>[2x]MRKHPQTATKHLFVSGGVASSLGKGLTASSLGQLLTARGLHVTMQKLDPYLNVDPGTMNPFQHGEVFVTEDGAETDLDVGHYERFLDRNLPGSANVTTGQVYSTVIAKERRGEYLGDTVQVIPHITDEIKRRILAMAQPDADGNRPDVVITEIGGTVGDIESQPFLEAARQVRHYLGREDVFFLHVSLVPYLAPSGELKTKPTQHSVAALRSIGITPDALILRCDRDVPEALKNKIALMCDVDIDGVISTPDAPSIYDIPKVLHREELDAFVVRRLNLPFRDVDWTEWDDLLRRVHEPHETVRIALVGKYVELSDAYLSVAEALRAGGFKHRAKVEICWVASDGCETTSGAAAALGDVHGVLIPGGFGIRGIEGKIGAIAYARARGLPVLGLCLGLQCIVIEAARSVGLTNANSAEFDPDTPDPVIATMPDQEEIVAGEADLGGTMRLGSYPAVLEPDSVVAQAYQTTQVSERHRHRYEVNNAYRDKIAESGLRFSGTSPDGHLVEFVEYPPDRHPFVVGTQAHPELKSRPTRPHPLFVAFVGAAIDYKAGELLPVEIPEIPEHTPNGSSHRDGVGQPLPEPASRG

The combined data indicate that 7947882 and 7904688 are prodrugs activated by the EthA monooxygenase, which then target PyrG, a cytidine triphosphate (CTP) synthetase catalyzing the ATP-dependent amination of uridine triphosphate (UTP) to form the essential pyrimidine nucleotide CTP. The crystal structure of PyrG was solved by molecular replacement on a 2.0-Å resolution data set. This structure showed a bidomain enzyme with an N-terminal amidoligase (ALase) domain, also commonly known as the synthetase domain (residues 1–278), connected through an interdomain linker (residues 279–Pro298) to a C-terminal glutamine amidotransferase (GATase) domain (residues 299–552), both domains displaying a Rossmann-like fold. On the other hand, the 34-residue C-terminal extension of M. tuberculosis PyrG, which has no predicted secondary structure or known function, could not be traced due to the lack of supporting electron density, suggesting a high degree of flexibility.

The enzyme, in complex with either UTP, at 2.0-Å resolution, or UTP plus the non-hydrolyzable ATP analog AMP-PCP and the glutamine analog 5-oxo-L-norleucine (3.5 Å), is a homotetramer with crystallographic 222 symmetry, consistent with previous studies reporting positive cooperativity for ATP and UTP due to nucleotide-driven tetramerization. In contrast, in the independent crystal form, grown in the presence of AMP-PCP as well as UTP and the glutamine analog 6-diazo-5-oxo-L-norleucine (L-DON), AMP-PCP lies in the ATP-binding site, as expected, with UTP maintaining the same orientation as above. In addition, a covalent adduct was observed between the Cys393 sulfur and oxonorleucine, as expected from the reaction with L-DON, therefore confirming the role of Cys393 as the catalytic nucleophile within a Gln-hydrolyzing triad that includes His524 and Glu526. In agreement with similar observations made on E. coli PyrG (Endrizzi et al., 2004), a putative ammonia diffusion channel was visualized connecting the glutaminase active site in the C-terminal domain to the synthetase site at the N-terminal domain. However, the tunnel is not continuous, but appears to be blocked by the side chains of residues Pro55, Pro60, and Val66, all located on the long β2 to β3 linker that includes the short α2, forming a constriction in the channel. The residue Val186 mutated to Gly in the M. tuberculosis-resistant mutants lies on the β7 strand behind the conserved P loop (Gly16 to Gly25) that contributes to bind the ATP phosphates, its side chain being at closest ∼7 Å from the AMP-PCP β-phosphate. Despite being located in the proximity of the ATP-binding pocket, the Val186Gly substitution does not provide any obvious explanation for the resistance profile to an ATP competitive inhibitor. Moreover, this mutation should have a destabilizing effect on the P loop and on its proper positioning within the ATP-binding cleft, leading to a decreased affinity for ATP.> MAEIVLDRVTKSYPDGAGGVRAAVKEFSMTIADGEFIILVGPSGCGKSTTLNMIAGLEEITSGELRIGGERVNEKAPKDRDIAMVFQSYALYPHMTVRQNIAFPLTLAKVPKAEIAAKVEETAKILDLSELLDRKPGQLSGGQRQRVAMGRAIVRSPKAFLMDQPLSNLDAKLRVQMRAEISRLQDRLGTTTVYVTHDQTEAMTLGDRVVVMLAGEVQQIGTP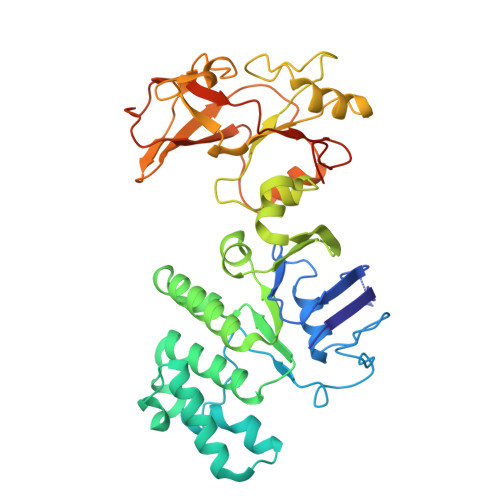DELYSSPANLFVAGFIGSPAMNFFPATRTDVGVRLPFGEVTLTPHMLDLLDKQARPENIIVGIRPEHIEDSALLDGYARIRALTFSVRADIVESLGADKYVHFTTEGAGAESAQLAELAADSGAGTNQFIARVSADSRVRTGEQIELAIDTTKLSIFDAATGLNLTRDITPTDPTEAAGPDAG> MKRGFARPTPEKPPVIKPENIVLSTPLSIPPPEGKPWWLIVVGVVVVGLLGGMVAMVFASGSHVFGGIGSIFPLFMMVGIMMMMFRGMGGGQQQMSRPKLDAMRAQFMLMLDMLRETAQESADSMDANYRWFHPAPNTLAAAVGSPRMWERKPDGKDLNFGVVRVGVGMTRPEVTWGEPQNMPTDIELEPVTGKALQEFGRYQSVVYNLPKMVSLLVEPWYALVGEREQVLGLMRAIICQLAFSHGPDHVQMIVVSSDLDQWDWVKWLPHFGDSRRHDAAGNARMVYTSVREFAAEQAELFAGRGSFTPRHASSSAQTPTPHTVIIADVDDPQWEYVISAEGVDGVTFFDLTGSSMWTDIPERKLQFDKTGVIEALPRDRDTWMVIDDKAWFFALTDQVSIAEAEEFAQKLAQWRLAEAYEEIGQRVAHIGARDILSYYGIDDPGNIDFDSLWASRTDTMGRSRLRAPFGNRSDNGELLFLDMKSLDEGGDG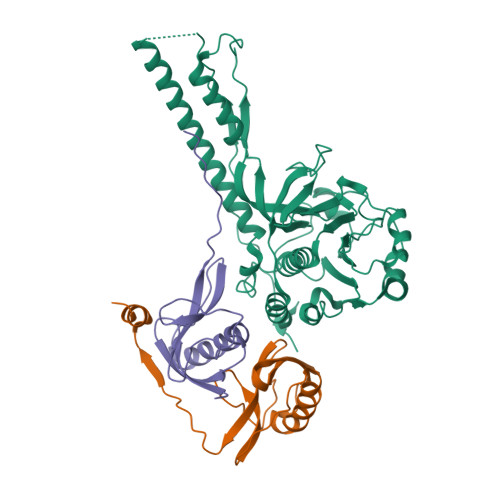PHGVMSGTTGSGKSTLVRTVIESLMLSHPPEELQFVLADLKGGSAVKPFAGVPHVSRIITDLEEDQALMERFLDALWGEIARRKAICDSAGVDDAKEYNSVRARMRARGQDMAPLPMLVVVIDEFYEWFRIMPTAVDVLDSIGRQGRAYWIHLMMASQTIESRAEKLMENMGYRLVLKARTAGAAQAAGVPNAVNLPAQAGLGYFRKSLEDIIRFQAEFLWRDYFQPGVSIDGEEAPALVHSIDYIRPQLFTNSFTPLEVSVGGPDIEPVVAQPNGEVLESDDIEGGEDEDEEGVRTPKVGTVIIDQLRKIKFEPYRLWQPPLTQPVAIDDLVNRFLGRPWHKEYGSACNLVFPIGIIDRPYKHDQPPWTVDTSGPGANVLILGAGGSGKTTALQTLICSAALTHTPQQVQFYCLAYSSTALTTVSRIPHVGEVAGPTDPYGVRRTVAELLALVRERKRSFLECGIASMEMFRRRKFGGEAGPVPDDGFGDVYLVIDNYRALAEENEVLIEQVNVIINQGPSFGVHVVVTADRESELRPPVRSGFGSRIELRLAAVEDAKLVRSRFAKDVPVKPGRGMVAVNYVRLDSDPQAGLHTLVARPALGSTPDNVFECDSVVAAVSRLTSAQAPPVRRLPARFGVEQVRELASRDTRQGVGAGGIAWAISELDLAPVYLNFAENSHLMVTGRRECGRTTTLATIMSEIGRLYAPGASSAPPPAPGRPSAQVWLVDPRRQLLTALGSDYVERFAYNLDGVVAMMGELAAALAGREPPPGLSAEELLSRSWWSGPEIFLIVDDIQQLPPGFDSPLHKAVPFVNRAADVGLHVIVTRTFGGWSSAGSDPMLRALHQANAPLLVMDADPDEGFIRGKMKGGPLPRGRGLLMAEDTGVFVQVAATEVRR;>[2x]MTAVADAPQADIEGVASPQAVVVGVMAGEGVQIGVLLDANAPVSVMTDPLLKVVNSRLRELGEAPLEATGRGRWALCLVDGAPLRATQSLTEQDVYDGDRLWIRFIADTERRSQVIEHISTAVASDLSKRFARIDPIVAVQVGASMVATGVVLATGVLGWWRWHHNTWLTTIYTAVIGVLVLAVAMLLLMRAKTDADRRVADIMLMSAIMPVTVAAAAAPPGPVGSPQAVLGFGVLTVAAALALRFTGRRLGIYTTIVIIGALTMLAALARMVAATSAVTLLSSLLLICVVAYHAAPALSRRLAGIRLPVFPSATSRWVFEARPDLPTTVVVSGGSAPVLEGPSSVRDVLLQAERARSFLSGLLTGLGVMVVVCMTSLCDPHTGQRWLPLILAGFTSGFLLLRGRSYVDRWQSITLAGTAVIIAAAVCVRYALELSSPLAVSIVAAILVLLPAAGMAAAAHVPHTIYSPLFRKFVEWIEYLCLMPIFPLALWLMNVYAAIRYR> TEAAAQPHALPADAPDIAPERDLLSKFDGLIAERQKLLDSGVTDPFAIVMEQVKSPTEAVIRGKDTILLGTYNYMGMTFDPDVIAAGKEALEKFGSGTWGSRMLNGTFHDHMEVEQALRDFYGTTGAIVFSTGYMANLGIISTLAGKGEYVILDADSHASIYDGCQQGNAEIVRFRHNSVEDLDKRLGRLPKEPAKLVVLEGVYSMLGDIAPLKEMVAVAKKHGAMVLVDEAHSMGFFGPNGRGVYEAQGLEGQIDFVVGTFSKSVGTVGGFVVSNHPKFEAVRLACRP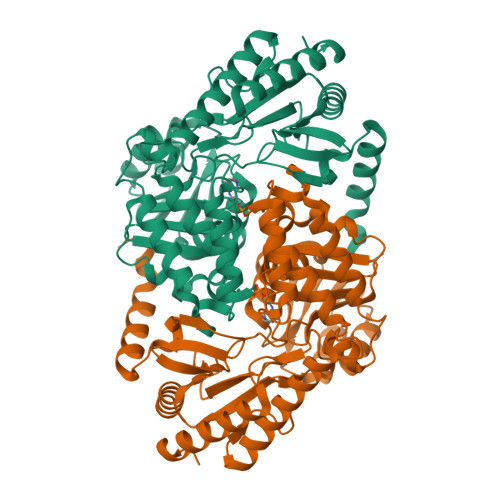YIFTASLPPSVVATATTSIRKLMTAHEKRERLWSNARALHGGLKAMGFRLGTETCDSAIVAVMLEDQEQAAMMWQALLDGGLYVNMARPPATPAGTFLLRCSICAEHTPAQIQTVLGMFQAAGRAVGVIGLEHHHHHH Virus ΦcrAss001 (Kehishuvirus primarius) was the first representative of this order to be isolated in pure culture from human faecal samples. Here, we present the characterization of ΦcrAss001 using cryo-electron microscopy (cryo-EM), enabling de novo structure building and elucidation of functions for around 1,440 protein subunits constituting the virion, leading to the identification of a novel ‘crass fold’ in the distal part of the tail. The virion possesses a short non-contractile tail extending approximately 44 nm from an icosahedral capsid. The extended tail barrel formed by widely conserved paralogous ring proteins has a high capacity for storage of cargo proteins alongside the capsid cargo zone, ensuring that the proteins required for the initial stages of crassvirus infection are carried inside virions and delivered to the host cell.

The barrel was reconstructed by imposing C12 symmetry to a resolution of 3.20 Å, and with C6 symmetry to a resolution of 3.30 Å. The barrel is composed of five stacked dodecameric ‘rings’, termed ring 1 (R1, at the portal end) to ring 5 (R5, at the muzzle end). These structures are formed by four paralogous ring proteins: R1, R2 and R3 are encoded by genes gp43, gp40 and gp35, respectively, whereas R4 and R5 are both encoded by gp34. The ring proteins share highly similar folds and consist of two domains, with three structurally conserved α-helices and a β-sandwich domain. R1 and R2 form an interface for interaction with the tail fibre docking hubs, which are the point of attachment of the tail fibre appendages. The tail hub (TH) proteins form a continuous ‘collar’ around the tail barrel. Each hub assembly is an A2B trimer that consists of two copies of THA (gp38) and one copy of the smaller protein THB (gp39). The C-terminal segment of THB, residues 67–107, extends into the neighbouring hub, resulting in continuous interlocking ring of 12 docking hubs around the barrel. Each docking hub, in turn, interacts with the trimeric tail fibre protein gp22, accommodating its N-terminal residues 1–26. Unexpectedly, well-defined density at the inner surface of R1 and R2 of the tail barrel corresponds to 12 copies of an additional α-helical segment of the same protein, gp45 (residues 214–245).

> MADFLNFPRQMLPFSKKTKQWRKDCLLWANQKTFFNYSLVRKSVIHKKINYDLLNGRLHMSDLELVLNPDGIKAAYIPDRLQHYPIMNSKLNVLRGEESKRVFDFKVVVTNPNAISEIEDNKKNELLQRLQEMITDTSISEDEYNIKLEKLNDYYTYEWQDIREVRANELLNHYIKEYDIPLIFNNGFMDAMTCGEEIYQCDIVGGEPVIERVNPLKIRIFKSGYSNKVEDADMIILEDYWSPGRVIDTYYDVLSPKDIKYIETMPDYIGQGAVDQMDNIDERYGFVNQNMIGDEITVRDGTYFFDPANLFTEGIANSLLPYDLAGNLRVLRLYWKSKRKILKVKSYDPETGEEEWNFYPENYVVNKEAGEEVQSFWVNEAWEGTMIGNEIFVNMRPRLIQYNRLNNPSRCHFGIVGSIYNLNDSRPFSLVDMMKPYNYLYDAIHDRLNKAIASNWGSILELDLSKVPKGWDVGKWMYYARVNHIAVIDSFKEGTIGASTGKLAGALNNAGKGMIETNIGNYIQQQINLLEFIKMEMADVAGISKQREGQISQRETVGGVERATLQSSHITEWLFTIHDDVKKRALECFLETAKVALKGRNKKFQYILSDTSTRVMEIDGDEFAEADYGLVVDNSNGTQELQQKLDTLAQAALQTQTLSFSTITKLYTSSSLAEKQRLIEKDEKQIRERQAQAQKEQLEAQQQIAAMQQQQKEAELLQKEEANIRDNQTKIIIAQIQSEGGPDEEDGIMIDDYSPEAKANLAEKIREFDEKLKLDKDKLKLDKKKAETDASIKRQALRKKSSTTNK;> MVNNINWVKLPVILDRLLRHPLLTDLNLETAIQYTLDFISAMGLPNVYVDKIETIDIKEYRGELPCDLISINQVRLHKNGIALRAMTDNFNAYPTHDHKEGDWYERGEPSFKTQGRVIFTSIKHEKVDISYKAIMLDDEGLPLIPDNPIFLKTLELYIKKEWFTILFDMGKISPAVLNNTQQEYAFKAGQCNNEFVIPSVSEMEAITNMWNQLIPRVTEFRRGFKNLGDKEYIRVH;> MTYNELIYMVLDELKLSSDDSYYTPDHVIFLLVKYRSFLLKQRYSDIKKQIPDSDYQSICLDLIEVPAISGEPCEGSSYLRSKNKVPTTMMIGNPRVYPMDFYQGEITYISRDRMRYVGYNKFLRNIIYCSKAPDGYLYFKSWNPQFLHLEKVSFNAIFEDAKEASEMACPEENGTICKLEDKEFPIEDALVPPLIELVVKELRGPEYSPKDEDNNAKDDLPDAR;> MTNKEFSDGFSTLLNSFGITPNITLDEYEKSTFLTNAQEQLIIDIYSGRNIIYGKSFEQTEEIRRYLSNLVETYETSTKVTGKLGLSKDSVFFEIPQDTWFITYEVAFLKDSRLGCLDGIEASVVPLPQDDLYRAKDNPFRGPSKDRVLRLDIKSDLAELISKYNVDKYLMRYISQPTPIILVDLPDGLSINGVSTESECELNPVVHRAILERAVQLAIISKTQLTGNKE;>[2x]MNVNEFSNEFDVLYNNIMSNAAPGLNEYEKSVLLTKAQEEIVKNYFEPAGNKYGKGLDDSPKRQIDFSELIKVGEGVLNTSAPTITFDKRAKVYDLPADLFLVINEAVDTNAGTKQIVPISYSDYTRLMSRPYKEPVKYQAWRIITTSINNISVELIVNSNETITDYKVRYIRRPAPIITTNLSSEYGDVTINGVSTVSECELNPIIHSEILQRAVELAKAAYQGDLQASVELGQRSE;>[2x]MHFNELRISQDNRFLIIDVSVDNQDYFEDVLLDSIVIDTQDTFVMNGPSDNPLYIYNVEDAYDLTYSLPEQCNCNPVRVEEDESYCFTYGTQQMKNVRLELNIQDLKVSPCSTMFFVYVKSKGTPSTDTPCGFDKDQILGTVINLQPIYKQTLKYLKEVECDCNIPKGFIDMILKLKAIELCVRTGNYPQAIKYWNKFFIKNNCKSPTSNCGCYG;> MDKMLEISEEAITRYFTTLSQFGYKKYSDVDKIIVLFFMEEMLAGEMSYYVTQDDYRNIVNALYCLAGSTCMIDFPMFESYDTLVHSNNRTFVPRITEDSILRSTEDDNFRVEA;>MFFTQEDYRKIEKWLLANSRKDTDFAGAATPLKGNETVVLVQNGKNVKASVKDVVEQLFLLGVSDFVNITDKYGESYISLSQAIELIPYRSRKIGQVVTFLDDTGKWAMFQFQGTRKNQWGTLSLWVDLIDLMTGLTITDSEDIVTETNSANQVALKFADKTYNEADYSGLGRVYLRKNIVNVEDPVTGNIVKMNYLTQSMISKENTIYIVQYSYNLNGQTITIPSGCVLKFEGGSISNGSIKGTDTNIIAPQIRIFNTILLSGTWKVRDIFDDWFDFNATTNFDNINNFYNISILQSDDLENNVILKGNYYSSLKDGIVLSLSSNTNLVLNGSISLLPNNLSSYSIIKGVDKENIKISGGGRLIGDLQNHLGDTGEWGFGISFTGCKTVSITNIDSSYMWGDGLYIGASDDTKEETLSQNIQVNNCKFEYNRRQGISITGAVDVFVNNCYFFNTGKINGTSPKAGLDIEPSGLYNSNVTISNCIADSNVSTGFLVYGDNRNIVIDNCASKNQLISITIAQRSATTDNDDVFIRHGNIGGSLQITRGNIRVEDCEVDSVYFTADTSGIGANVTISNSVIGAKRWEGSTYFNSVFLIDSNSQINNLYIFDSKIDYDPSILTQGLFNIGGNSIRDNILFENCDISQKNTVNSLNTKVGSYRNCRFYNMTRIYLANEPNKTVEFTDNYCAMTRESSSTNIFSFLNSSSTQDVILFVVRNNTFSTKGSINVGSIGLIDVTGVNLGNKMIFENNHFLTQYPLTQEQIIKALSNRITVDTNYNFTSRFPYRATLESLPAYNTFDAGALIYGDDNLLYFWNGTNLTNSEGTDARKVVIV[3x];>MAKKKIKRRGKMPPNIFDTGGQSWGQQSSGQFSNAFKGENLGNSIGSIGGAVGGIAQAGISNAQIADTSGIEAQNKAQKNMVVGASSNDDLMSEWGSWNKVKDDYSWKDVRGGSTGQRVTNTIGAAGQGAAAGASVGGPIGAIVGGVVGLGSAIGGWLGGNRKAKRKAKKLNKEAKEANERALTSFETRADNIDTQNDFNMLANFSAYGGPLEFGSGAIGYEFDNRYLNNQEMSAVAKQRLTSLPNSFQALPEMNTYNAFAEGGGLSREKNYGSKKKPYPSVPSGDFAGPHRSYPIPTKADARDALRLAGLHGNESVRRKVLAKYPSLKAFGGSLFDSVVGNNFNQSFTQGIQGMFQQEPEQTVQAANIAKDGGDIKIKEKNKGKFTAYCGGKVTEACIRKGKNSSNPTTRKRATFAQNARNWNAFGGWLNTQGGDFTNGVTFINEGGSHEENPYQGIQIGVDPEGAPNLVEQGEVVYDDYVFSDRMEIPDDIRKEYKLRGKTFAKAAKSAQRESEERPNDPLSTKGLQAAMERIATAQEEARQRKEAHREGNEYPSMFAYGGDTNPYGLALEDPMSVEELEALMVQSGETGEIAPEGNNGNRQTWTRYAPIIGSGLASLSDLFSKPDYDSADLISGVDLGAEAVGYAPIGNYLSYRPLDRDFYINKMNQQAAATRRGLMNTSGGNRLNAQAGILAADYNYGQNMGNLARQAEEYNQQLRERVEAFNRGTNMFNTETGLKASMFNAESRNAAKRARLGQATTVAQLRQGIKDQDAARRSANITNFLQGLGDMGWENEQANWLDTLAKSGVLKMNTKGEYTGGTKKAKGGKVRTKKKKGLTYG[2x]2-methyl-N-(2-sulfanylethyl)-1-benzofuran-3-carboxamide | 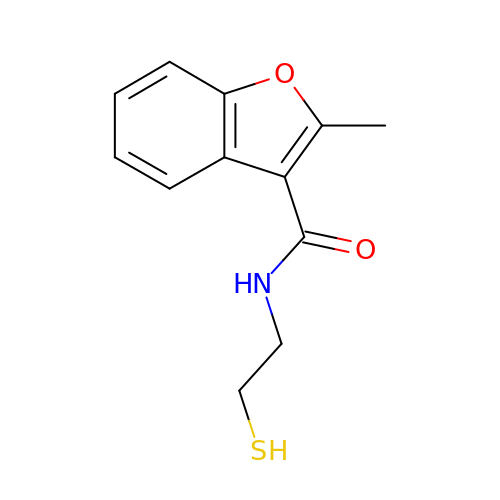C12 H13 N O2 S | MMIVKJYKVVAJCP-UHFFFAOYSA-N αD-conotoxins are 11 kDa homodimers that potently inhibit nicotinic acetylcholine receptors (nAChRs) through a non-competitive (allosteric) mechanism. VxXXA, VxXXB, and VxXXC from the venom of Conus vexillum were the first D superfamily α-conotoxins characterized. αD-conotoxins are 11 kDa symmetrical homodimer proteins comprising two C-terminal domains (CTDs or C) coupled through two interchain disulfide bonds formed between the N-terminal domains (NTDs). AChBPs are naturally occurring soluble protein homologues of the nAChR that show remarkable structural homology, especially around the orthosteric ligand recognition site formed by aromatic side chain residues found in nAChRs. In this study, we describe the allosteric binding mode of the granulin-like C-terminal (CTD) of VxXXB bound to Lymnea stagnalis acetylcholine binding protein (Ls-AChBP), a soluble homologue of the extracellular ligand-binding domain of nAChRs.

The crystal structure of Ls-AChBP in complex with VxXXB-C (21–50) was solved at 2.6 Å by molecular replacement and refined to an Rfree value of 0.29. The crystal structure of Ls-AChBP in complex with VxXXB-C(21–50) contains one pentamer in the asymmetric unit, with the electron density of VxXXB-C(21–50) detectable adjacent to four of the five orthosteric binding sites. However, only three binding interfaces generated clear ligand electron density, while the fourth binding interface showed reduced electron density. The F-loops of Ls-AChBP could not be constructed due to the lack of clear electron density, indicating a greater flexibility of these parts of the protein. VxXXB-C(21–50) binds to the C-loop of AChBP almost perpendicular to the long axis of the pentamers, making extensive interactions on the principal (+) face of Ls-AChBP. As observed from the co-crystal structure, VxXXB-C(21–50) anchors on the outer edge of C-loop Ls-AChBP via four hydrogen bonds between its β-strand backbone and β-strand of Ls-AChBP_C-loop and β4-loop inserting into the binding interface. In the four occupied orthosteric binding sites, loop-C of Ls-AChBP moves outward (10.23–10.90 Å based on the measurement between Cys187 Cα atom in the complex with HEPES/Ls-AChBP structure), which is a similar backbone orientation to previously characterized co-crystal structures of α-conotoxins 14–17. An outward displacement of Ls-AChBP_C-loop, which is characteristic of antagonist binding in the orthosteric site, is also displayed by VxXXB-C(21–50), suggesting allosteric antagonists can also inhibit nAChRs by stabilizing the open (extended) C-loop.

>[5x]LDRADILYNIRQTSRPDVIPTQRDRPVAVSVSLKFINILEVNEITNEVDVVFWQQTTWSDRTLAWNSSHSPDQVSVPISSLWVPDLAAYNAISKPEVLTPQLARVVSDGEVLYMPSIRQRFSCDVSGVDTESGATCRIKIGSWTHHSREISVDPTTENSDDSEYFSQYSRFEILDVTQKKNSVTYSCCPEAYEDVEVSLNFRKKG;>[3x]TRMCGSMSCPRNGCTCVYHWRRGHGCSCPG S. cerevisiae Pdr6/Kap122 was originally identified as a pleiotropic drug–resistance protein and subsequently as an importin β superfamily member. Furthermore, we found that Pdr6 imports Ubc9, exports eIF5A, and thus, combines functions of Imp13 and Xpo4. Pdr6 is an all α-helical protein built of 19 canonical HEAT repeats followed by three helices (termed HEAT 20) at its very C-terminal region. The transport signals recognized by Pdr6 are folded domains.

Diffracting Ubc9-bound Pdr6 crystals were obtained from a complex comprising full-length S. cerevisiae Ubc9 and Pdr6 proteins. Pdr6 binds Ubc9 in an open superhelix conformation. In the import complex, Pdr6 adopts an open conformation where the distance between the tip of HEAT 20 and the loop between HEATs 4 and 5 is ∼25 Å. Ubc9 is bound to the inner surface of the superhelix with HEATs 6–18 of Pdr6 engaging in extensive interactions with Ubc9. The first interaction interface is formed by residues of HEATs 6–9 and involves mostly salt bridges. Several aspartic acid residues of Pdr6 at this region (D370, D429, D433, D436, D492, and D499) form a negatively charged patch, shielding the conserved basic residues at the helix α1, as well as the following loop and two β-strands of Ubc9. The second set of interactions involves HEATs 11–18 of Pdr6. Helices α4 and α3 of Ubc9 pack against HEATs 12–15 and HEATs 16–17, respectively. Overall, Pdr6 buries 1,473 Å2 of the Ubc9 surface area. Our structure of the Ubc9•Pdr6 import complex revealed that Pdr6 is transporting Ubc9 in an inhibited state with blocked interaction sites for the E1 SUMO-activating enzyme with SUMO E3 ligases and SUMOylation substrates.

> SSIHEVVALIEELYSPHPKHDVNQIQQSLQSIQKSEQGFHLANELLSDDKYSANVKYFGALTLTVQLNTRGENDYETLWNVFRSNLLYLTKFSTLYVSNPNMYGQSLIIIKKLMSNLSLIFTKINDPQLNNAGNENMIKQWNNPINTFIQLMSVQNQNINADQLLLDSINCSLTYEQLSQFVSLSQKHNELALTFTEVIVEDLTKFQTKRHSMSQIHEVVHEHLYISTMALINLNLTAQAVFNPTVFDCITAWINYISLTRSVSSSGRMDLSEIFQNLIDLMYQSTEGSDGYENAEKILTIFGNVFANDPLLMSYDLRQQIECIFLGVVRPDSGITDISNKNSWMLQYMNYLVTNDFFSELKELAICIVDFLQINTLSVCNKLFTNIQAADNGQVQDEYIQEYIKVLLQMTNFPLTPVLQEFFSVRMVDFWLDLSDAYTNLASETLRPNSIELSTQIFQQLINIYLPKISLSVKQRIIEEEGESTSVNEFEDFRNAVSDLAQSLWSILGNDNLTNVLIDGMGQMPAASDETLIIKDTDVLFRIETMCFVLNTILVDMTLSESPWIKNIVDANKFFNQNVISVFQTGFQTSASTKVSQILKLDFVRTSTTLIGTLAGYFKQEPFQLNPYVEALFQGLHTCTNFTSKNEQEKISNDKLEVMVIKTVSTLCETCREELTPYLMHFISFLNTVIMPDSNVSHFTRTKLVRSIGYVVQCQVSNGPEEQAKYILQLTNLLSGSIEHCLASSVQLQEQQDYINCLLYCISELATSLIQPTEIIENDALLQRLSEFQSFWSSDPLQIRSKIMCTIDKVLDNSIYCKNSAFVEIGCLIVGKGLNLPDGEPYFLKYNMSEVMNFVLRHVPNCELATCLPYFVYLLEKLISEFRKELTPQEFDFMFEKILLVYYDAYIINDPDLLQMTIGFVNNVLDVKPGLAIGSKHWTSFILPQFLKLIPSREKFTIVAVAKFWTKLINNKKYNQEELTTVRQQVSSIGGDLVYQIMYGLFHTQRSDLNSYTDLLRALVAKFPIEAREWLVAVLPQICNNPAGHEKFINKLLITRGSRAAGNVILQWWLDCTTLPNYQG;> GSSLCLQRLQEERKKWRKDHPFGFYAKPVKKADGSMDLQKWEAGIPGKEGTNWAGGVYPITVEYPNEYPSKPPKVKFPAGFYHPNVYPSGTICLSILNEDQDWRPAITLKQIVLGVQDLLDSPNPNSPAQEPAWRSFSRNKAEYDKKVLLQAKQYSK> IINGEDCSPHSQPWQAALVMENELFCSGVLVHPQWVLSAAHCFQNSYTIGLGLHSLEADQEPGSQMVEASLSVRHPEYNRPLLANDLMLIKLDESVSESDTIRSISIASQCPTAGNSCLVSGWGLLANGRMPTVL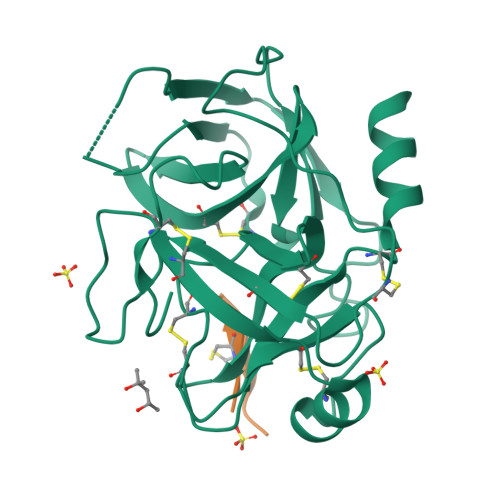QCVNVSVVSEEVCSKLYDPLYHPSMFCAGGGQDQKDSCNGDSGGPLICNGYLQGLVSFGKAPCGQVGVPGVYTNLCKFTEWIEKTVQA;> GFCQRSIPPICFPN>HHHHHHGSMNLTIIGSGKVGLVTGACLADIGHDVFCLDVDQAKIDILNNGGVPIHEPGLKEVIARNRSAGRLRFSTDIEAAVAHGDVQFIAVGTPPDEDGSADLQYVLAAARNIGRYMTGFKVIVDKSTVPVGTAERVRAAVAEELAKRGGDQMFSVVSNPEFLKEGAAVDDFTRPDRIVIGCDDDVPGERARELMKKLYAPFNRNHERTLYMDVRSAEFTKYAANAMLATRISFMNELANLADRFGADIEAVRRGIGSDPRIGYHFLYAGCGYGGSCFPKDVEALIRTADEHGQSLQILKAVSSVNATQKRVLADKIVARFGEDLTGRTFAIWGLAFKPNTDDMREAPSRELIAELLSRGARIAAYDPVAQEEARRVIALDLADHPSWLERLSFVDDEAQAARDADALVIVTEWKIFKSPD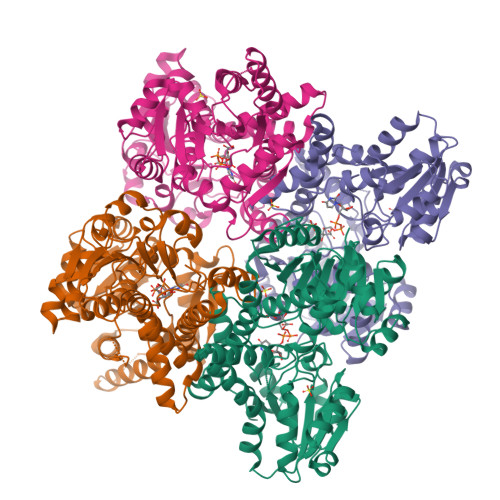FVALGRLWKTPVIFDGRNLYEPETMSEQGIEYHPIGRPGSRQAVAARVTGTAPASA[4x]> AANCADAAAAIVQAQWEDVWSAAAAAASRVSAGEEVFAALFKMVPAAKNLFTRVNVADINS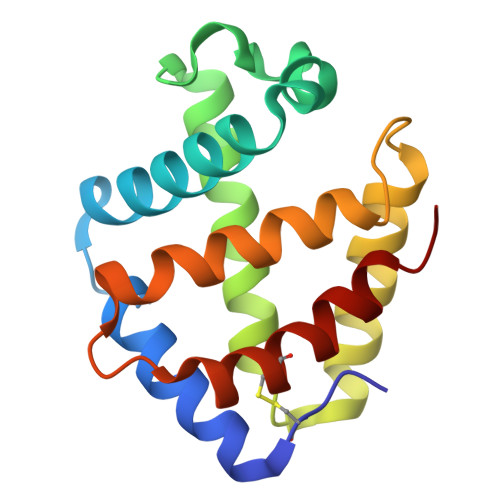PEFQGHVVRVMGGLDILINALDDIPTLESMLDHLAGQHAVRDGVTGAGFQLMATVLMESLPQVVEGFNPDAWASCLAGIAAAISSAL Rspo (R-spondin, also roof plate-specific spondin) proteins are evolutionarily conserved from fish to humans and have well-documented roles in a broad range of developmental and physiological processes resulting from enhancement of canonical and non-canonical Wnt signalling. ZNRF3/RNF43 specifically targets these Wnt receptors for ubiquitination and turnover, hence reducing Wnt signalling responses. Direct extracellular interaction with Rspo proteins inhibits ZNRF3/RNF43 activity. Here we report a molecular level analysis of the ZNRF3/RNF43 ectodomain structure and its interactions with Rspo proteins.

By using a combination of heavy atom and molecular-replacement-based phasing strategies, we determined multiple crystal structures for Xenopus (x) Rspo2Fu1–Fu2 (highest resolution 2.2 Å), xZNRF3ecto, zebrafish (z) ZNRF3ecto and mouse (m) ZNRF3ecto, (highest resolutions 2.4, 1.6 and 2.0 Å, respectively), plus complexes comprising xZNRF3ecto–xRspo2Fu1–Fu2, mZNRF3ecto–mRspo2Fu1–Fu2, mZNRF3ecto–xRspo2Fu1–Fu2 and xRNF4F3ecto–xRspo2Fu1–Fu2 (at 2.1, 2.8, 2.4 and 2.7 Å, respectively). The ZNRF3ecto crystal structures revealed a distinctive variant of the protease-associated domain topology. Two β-sheets (comprising β2, β1, β7, β3 and β4, β5, β6 strands, respectively) splay apart, accommodating an α-helix (αC) at the open edge; two additional α-helices (αA and αB) pack against the β4, β5 and β6 face of this distorted β-sandwich. A disulphide bridge, conserved across species, links two structurally elaborate loops, β3–β4 and β4–αA. The resultant single-domain structure is relatively compact. The crystal structures for apo xZNRF3ecto, zZNRF3ecto and mZNRF3ecto showed no major differences in the main chain conformation. Comparisons of ZNRF3ecto structures for proteins crystallized in several different crystal lattices, or for crystals containing multiple copies in the asymmetric unit, consistently highlighted an acidic region (N105-E114; residue numbering is for mouse sequences unless otherwise stated) within the β3–β4 loop, the short αC–β7 loop and the extended β1–β2 hairpin as flexible elements of the fold. Our crystallographic data provided independent structures for multiple copies of the ZNRF3 ectodomain in eight different crystal forms. All but two of these crystal structures reveal an extensive interface (average interface area 992±109 Å2) formed between two ZNRF3ecto polypeptide chains. The interaction is twofold symmetric; strands β3 and β7 of the ‘subunits’ abut face-to-face at the core of the dimer.

>[2x]ETGKDTAFVEVVLFESSPNGDYTTYTTGLQGRFSRAGATISAEGEIVQMHPLGLCNNNDEEDLYEYGWVGVVKLEQPELDPSCLTVLGKAKRAVQRGATAVIFDVSENPDAIDQLNQVSEDPLKRPVVYVKGADAVKLMNIVNKQKVARARIQHRGTKHHHHHH> MHHHHHHITSLYKKAGFMNKILESIRGKLIVSCQALEDEPLHSSFIMGRMAYAAYSGGAAGIRANTVEDIKEIKKNVSLPIIGIIKKVYNNSDVYITPTIKEVEDLINEGVQIIAIDATKRER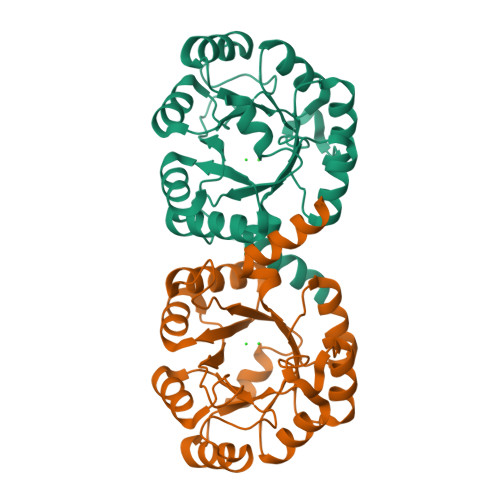PDRKDLKNFIAEIKEKYPNQLFMADISSVDEALYAEKIGFDIVGTTLVGYTDYTKNYKALEELKKVVKVVKIPVIAEGNIDTPLKAKKALEIGAFAVVVGGAITRPQQITKKFVDEMK> MRGSHHHHHHGSSQISRGLENVFIKTTSLTYIDGENGILRYGGYDIEDLVEHTSFEEVVHLMLYGDLPTKLQLQRLKSALDEAYEVPQQVIDMIYSLPRDSDAVGMMETAFSALSSIYGMPWNKATNRDNAVKLVARASTVVANVLRAKEGKKPAIPEPSESFAKSFLKASFSRTPTEEEVKAMDAALILYADHEVPASTTAALVTSSTLSDIYSCVVAALAALKGPLHGGAAEEAFKQFVEIGEPDMTESWFKRKIIEGKSRLMGFGHRVYKTYDPRAKIFKKYAKVISERNSDARKYFEI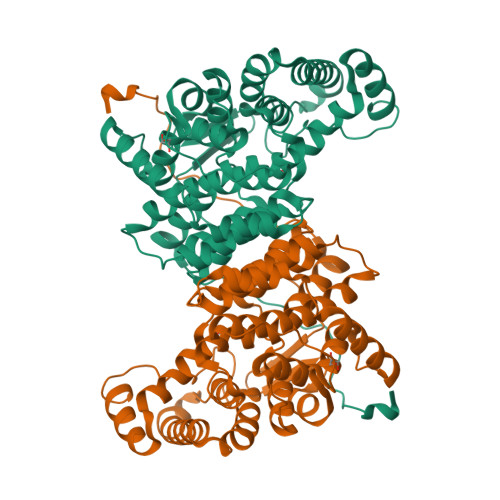AQKLEELGVETFGAKHIYPNTDFYSGVVFYALGFPVYMFTSLFALSRTLGWTAHVIEYVEDQHRLIRPRALYVGPLKRDVVPIELRG>MSAPTPLAEASQIPTIPALSPLTAKQSKGNFFSSNPISSFVVDTYKQLHSHRQSLELVNPGTVENLNKEVSRDVFLSQYFFTGLRADLNKAFSMNPAFQTSHTFSIGSQALPKYAFSALFANDNLFAQGNIDNDLSVSGRLNYGWDKKNISKVNLQISDGQPTMCQLEQDYQASDFSVNVKTLNPSFSEKGEFTGVAVASFLQSVTPQLALGLETLYSRTDGSAPGDAGVSYLTRYVSKKQDWIFSGQLQANGALIASLWRKVAQNVEAGIETTLQAGMVPITDPLMGTPIGIQPTVEGSTTIGAKYEYRQSVYRGTLDSNGKVACFLERKVLPTLSVLFCGEIDHFKNDTKIGCGLQFETAGNQELLMLQQGLDADGNPLQALPQLGGWSHPQFEK[4x];>MVELTEIKDDVVQLDEPQFSRNQAIVEEKASATNNDVVDDEDDSDSDFEDEFDENETLLDRIVALKDIVPPGKRQTISNFFGFTSSFVRNAFTKSGNLAWTLTTTALLLGVPLSLSILAEQQLIEMEKTFDLQSDANNILAQGEKDAAATANGGHHHHHHHH[4x];>MFGLPQQEVSEEEKRAHQEQTEKTLKQAAYVAAFLWVSPMIWHLVKKQWK[4x];>MDGMFAMPGAAAGAASPQQPKSRFQAFKESPLYTIALNGAFFVAGVAFIQSPLMDMLAPQL[4x];>MSFLPSFILSDESKERISKILTLTHNVAHYGWIPFVLYLGWAHTSNRPNFLNLLSPLPSV[4x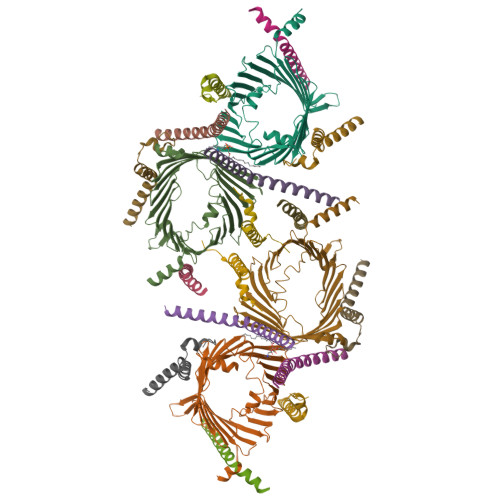]>SNAMLISVLKSKISYATVTGKDLFYVGSITIDSEIMKQANIIENEKVQVVNLNNGERLETYVIKGEPNSKT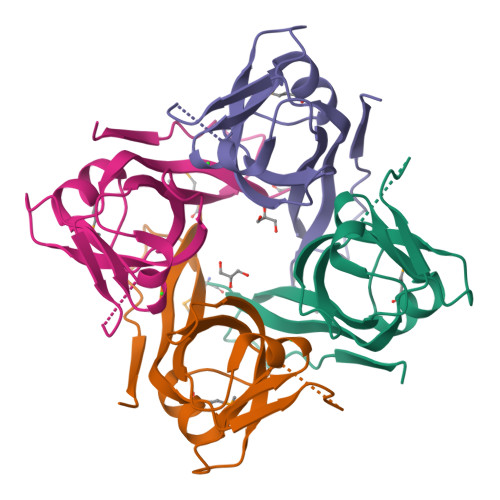IALNGPAARRCEIGDQLFIISYTQVDPTRENIKPKLVDLKTGD[8x]2-AMINO-3-{(1R)-1-CYCLOHEXYL-2-[(CYCLOHEXYLCARBONYL)AMINO]ETHYL}-6-PHENOXYQUINAZOLIN-3-IUM | C29 H37 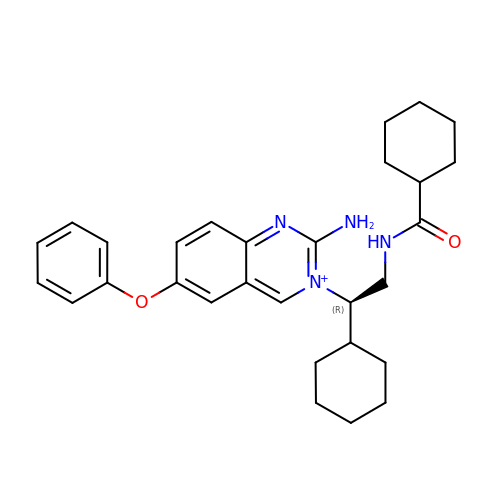N4 O2 | JJSGXQVHJOYNEC-MHZLTWQESA-O>GSSETSVNRGPEKIRPECFELLRVLGKGGYGKVFQVRKVTGANTGKIFAMKVLKKAMIVRNAKDTAHTKAERNILEEVKHPFIVDLIYAFQTGGKLYLILEYLSGGELFMQLEREGIFMEDTACFYLAEISMALGHLHQKGIIYRDLKPENIMLNHQGHVKLTDFGLCKESIHDGTVTHTFCGTIEYMAPEILMRSGH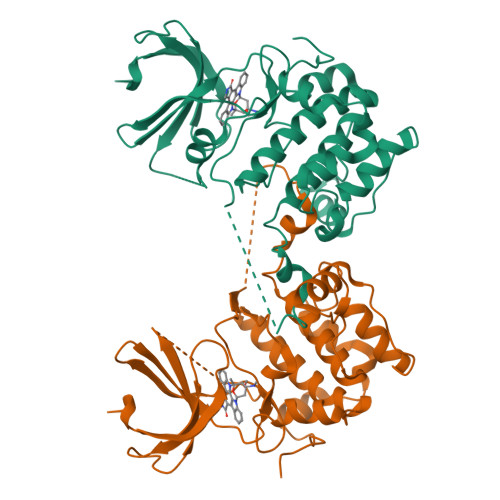NRAVDWWSLGALMYDMLTGAPPFTGENRKKTIDKILKCKLNLPPYLTQEARDLLKKLLKRNAASRLGAGPGDAGEVQAHPFFRHINWEELLARKVEPPFKPLLQSEEDVSQFDSKFTRQTPVDSPDDST[2x]>MRGSHHHHHHGSMPDLLTNVAENYVNQDLFAGIEWRIDQDGKPIFQGCAGVKDIETRTFIPKNAIYRIYSMTKPIVSFLAMMLIERGVFRLSSPIQNFDPRFKSMKVIDQHAHIEPATALITIEHLLTHQAGFSYDFSLGCPISAHYRDAQLIEDGGRDLTDMMGVLAELPLVFHPGTQWKYSISTDVLAHIIECATGERVDDLLQRLIFDPLDMQDTGFSLPLDGASRLMEVYGMRSLHGLPALKPAPHVLVPADLGSSHPTDD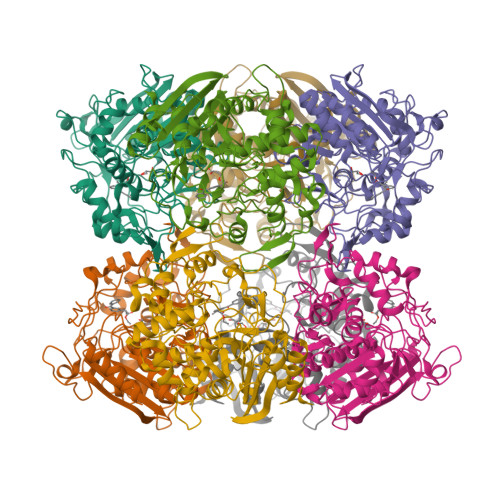PDFRRGGHGLYSTLDDYMAFANMLLSGQTPEGETLLSPAVLKLALAPRVHFGARGMRINDEPFAGYSWNLLGRVMTDVGAAAYATHLGEFGWSGVAATYFWVDPTKNMTGCVMTQFLGSQHPIGSDMQAAAMSMLG[2x]>[2x]MGSPDIE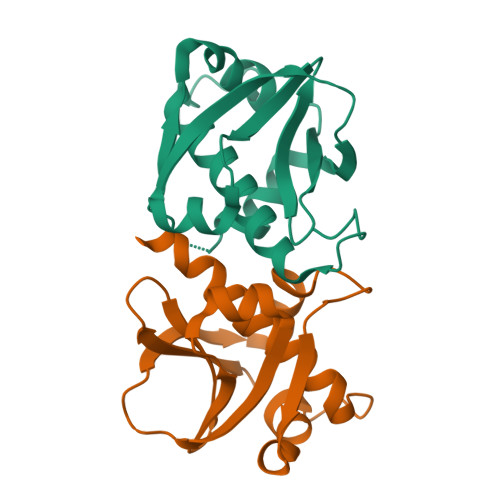LVYKNRGFYKHYGVRFGGHIYHLNSQDILSTAITGKSDFIKEEDDGKWVHAMTAPLDYFTEKYINSMVGSKHIFSATSNCETIARDLFPGRKEITQSKALGIIGVILLSASLLSLLAVPWDYSSLQTVYNQLEHHHHHH>[2x]SGSGSPELDE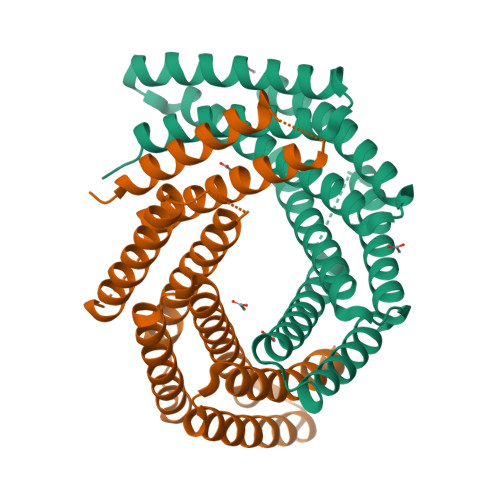LWKRVKKLVTELLEQAERAGDPEEIFKLLEVAQQLLWLAEMFLRLAAIQEKATDPEIQELAERVLRLIKRLLEEAERAGDPRRIKELVEVALALAKLLEMFYRLKEIQERATDPEIQELAERVLRLIKKLLKAAEEAGDPRKIYKLVFVALVLLHLLQTFYRLKEIQEKATDPEIQRKAQEVLEKIKRLLEAAERAGDPAKILLYVIRAQLLAMELKFAYRKR>MLFFNVASLKYKHHESIQMIIDRIDHLVLTVSDISTTIRFYEEVLGFSAVTFKQNRKALIFGAQKINLHQQEMEFEPKASRPTPGSADLCFITSTPINDVVSEILQAGISIVEGPVERTGATGEIMSIYIRDPDGNLIEIS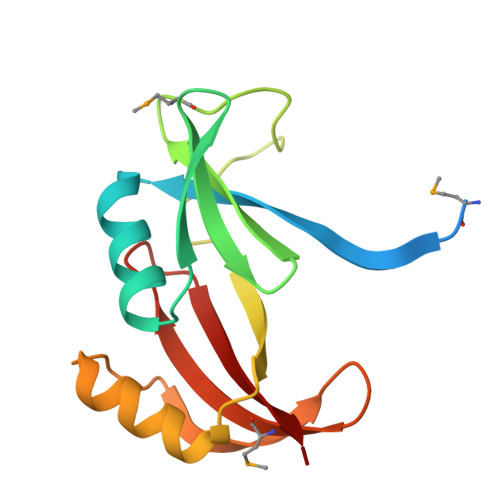QYV[4x]>MPVFDEPVYTVNVLENSPINTLVIDLNATDPDEGTNGEVVYSFINFVSNLTKQMFKIDPKTGVITVNGVLDHEELHIHEIDVQAKDLGPNSIPAHCKVIVNVIDINDNAPEIKLLSENSEMVEVSENAPLGYVIALVRVSDNDSGANGKVQCRLQGNVPFRLNEFESFSTLLVDGRLDREQRDMYNLTILAEDSGYPPLRSSKSFAVKVTDLEHHHHHH[4x]

Protocadherin-19 (PCDH19) is a member of the non-clustered δ2-protocadherin subfamily that is located on the X-chromosome. Mutations in PCDH19 cause an X-linked, female-limited form of infant-onset epilepsy (PCDH19 female epilepsy, PCDH19-FE; OMIM 300088) that is associated with intellectual disability, as well as compulsive or aggressive behavior and autistic features. However, PCDH19 along with the rest of the non-classical cadherins lack these critical tryptophan residues and must mediate adhesion by an alternative mechanism. Here we present crystals structures of the highly homologous zebrafish Protocadherin-19 (Pcdh19) encompassing repeats EC1-4 and EC3-4.

The solved structure for Pcdh19 EC3-4 (2.51 Å) includes four molecules in the asymmetric unit, each starting from Pro 213 and continuing to Asp 422 (numbering corresponds to the processed Danio rerio protein). Root-mean-square-deviation (RMSD) among these four molecules is <2.4 Å. The EC3-4 repeats from both structures superpose well (RMSD 2.1 Å), and good quality electron density maps allowed us to unambiguously position side chains for most residues. The final model for Pcdh19 EC3-4 is missing residues 243–246 in chain A, and residues 244–248 in chain B (chains C and D are complete). Pcdh19 EC3-4 was refolded by overnight dialysis against 20 mM TrisHCl [pH 7.5], 150 mM NaCl, 400 mM arginine, 2 mM CaCl2, 2 mM DTT using MWCO 2000 membranes. Crystals were grown by vapor diffusion at 4°C by mixing equal volumes of protein (Pcdh19 EC3-4 = 14.4 mg/ml and Pcdh19 EC1-4 = 7.7 mg/ml) and reservoir solution (Pcdh19 EC3-4 contained 100 mM calcium acetate, 100 mM sodium cacodylate [pH 6.1], 25% MPD; Pcdh19 EC1-4 contained 200 mM sodium chloride, 100 mM TrisHCl [pH 8.1], 8% PEG 20,000). Although the Pcdh19 EC3-4 structure does not reveal any relevant interface, the Pcdh19 EC1-4 structure does. The Pcdh19 EC3-4 N317S fragment refolded well as assessed by size exclusion chromatography (SEC), but its melting temperature is considerably lower (40.7 ± 0.6°C vs. 52.4 ± 0.3°C), even in the presence of 2 mM CaCl2. Another PCDH19-FE mutation of a surface residue (E313K, equivalent to E290K) did not show a dramatic shift in melting temperature (50.4 ± 0.1°C). These SEC and thermal stability results indicate that the EC3-4 fragment carrying the N317S mutation is folded, and may bind calcium, yet it is not as stable as the wild-type fragment.>[2x]MLEVPTDGNAGLLAEPQIAMFCGRLNMHMNVQNGKWDSDPSGTK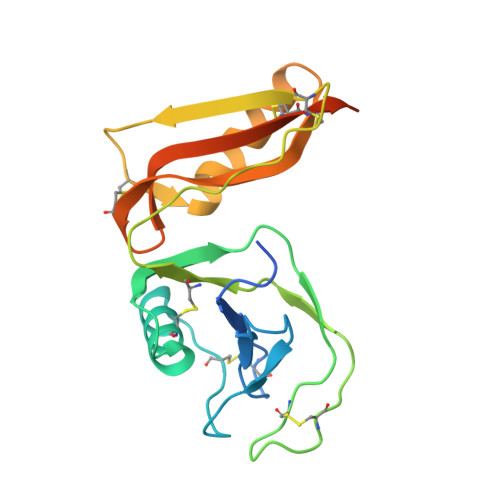TCIDTKEGILQYCQEVYPELQITNVVEANQPVTIQNWCKRGRKQCKTHPHFVIPYRCLVGEFVSDALLVPDKCKFLHQERMDVCETHLHWHTVAKETCSEKSTNLHDYGMLLPCGIDKFRGVEFVCCPLAIEGRKLAAALEHHHHHH>[2x]MFHGKHPGGLSERGRALLLEGGKALGLDLKPHLEAFSRLYALL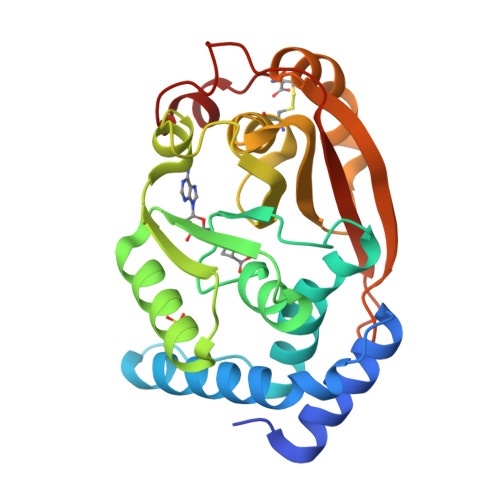QEASGKVNLTALRGEEEVVVKHFLDSLTLLRLPLWQGPLRVLDLGTGAGFPGLPLKIVRPELELVLVDATRKKVAFVERAIEVLGLKGARALWGRAEVLAREAGHREAYARAVARAVAPLCVLSELLLPFLEVGGAAVAMKGPRVEEELAPLPPALERLGGRLGEVLALQLPLSGEARHLVVLEKTAPTPPAYPRRPGVPERHPLC> MELLMIVVIGC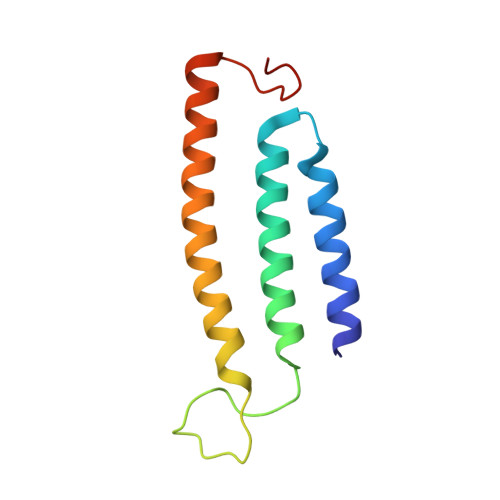LFAAATYLLLSKSLLRIIIGTGLLSHGAHLLLLTMGGLKAGAPPLLGEKASRYVDPLPQALILTAIVISFGVTAFFLVLAYRSYQEIGTDHMEGMKGD> GTIPKPTLWAEPDSVITQGSPVTLSCQGSLEAQEYRLYREKKSASWITRIRPELVKNGQFHIPSITWEHTGRYGCQYYSRARWSELSDPLVLVMTGAYPKPTLSAQPSPVVTSGG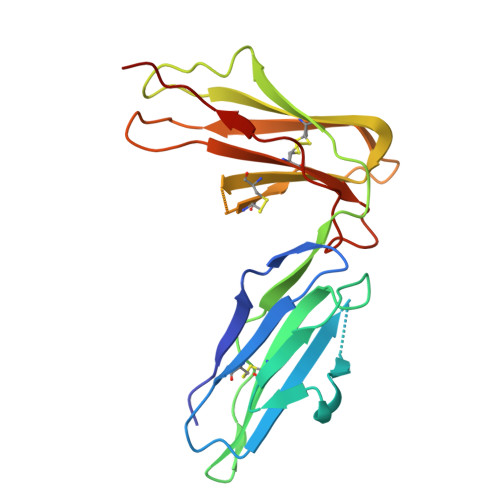RVTLQCESQVAFGGFILCKEGEDEHPQCLNSQPHARGSSRAIFSVGPVSPNRRWSHRCYGYDLNSPYVWSSPSDLLELLVPG>[2x]MAHHHHHHVTSLYKKAGSAAAPFTADTNSNVAVKQINNTGTNDSGEKKVPVPSTNNDSLKQGTDGFWYDSDGNRVDQKTNQILLTAEQLKKNNEKNLSVISDDTSKKDDENISKQTKIANQQTVDTAKGLTTSNLSDPITGGHYENHNGYFVYIDASGKQVTGLQNIDGNLQYFDDNGYQVKGSFRDVNGKHIYFDSVTGKASSNVDIVNGKAQGYDAQGNQLKKSYVADSSGQTYYFDGNGQPLIGLQTIDGNLQYFNQQGVQIKGGFQDVNNKRIYFAPNTGNAVANTEIINGKLQGRDANGNQVKNAFSKDVAGNTFYFDANGVMLTGLQTISGKTYYLDEQGHLRKNYAGTFNNQFMYFDADTGAGKTAIEYQFDQGLVSQSNENTPHNAAKSYDKSSFENVDGYLTADTWYRPTDILKNGDTWTASTETDMRPLLMTWWPDKQTQANYLNFMSSKGLGITTTYTAATSQKTLNDAAFVIQTAIEQQISLKKSTEWLRDAIDSFVKTQANWNKQTEDEAFDGLQWLQGGFLAYQDDSHRTPNTDSGNNRKLGRQPINIDGSKDTTDGKGSEFLLANDID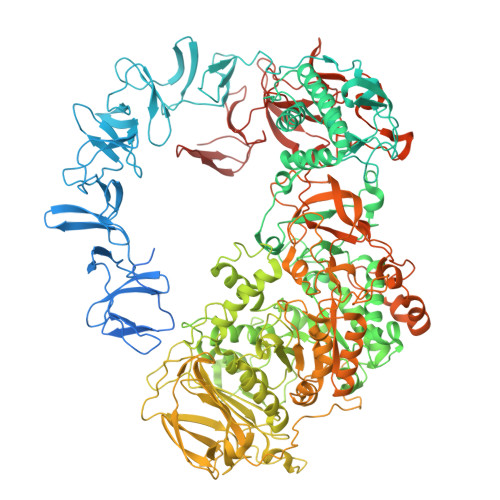NSNPIVQAEQLNWLHYLMNFGSITGNNDNANFDGIRVDAVDNVDADLLKIAGDYFKALYGTDKSDANANKHLSILEDWNGKDPQYVNQQGNAQLTMDYTVTSQFGNSLTHGANNRSNMWYFLDTGYYLNGDLNKKIVDKNRPNSGTLVNRIANSGDTKVIPNYSFVRAHDYDAQDPIRKAMIDHGIIKNMQDTFTFDQLAQGMEFYYKDQENPSGFKKYNDYNLPSAYAMLLTNKDTVPRVYYGDMYLEGGQYMEKGTIYNPVISALLKARIKYVSGGQTMATDSSGKDLKDGETDLLTSVRFGKGIMTSDQTTTQDNSQDYKNQGIGVIVGNNPDLKLNNDKTITLHMGKAHKNQLYRALVLSNDSGIDVYDSDDKAPTLRTNDNGDLIFHKTNTFVKQDGTIINYEMKGSLNALISGYLGVWVPVGASDSQDARTVATESSSSNDGSVFHSNAALDSNVIYEGFSNFQAMPTSPEQSTNVVIATKANLFKELGITSFELAPQYRSSGDTNYGGMSFLDSFLNNGYAFTDRYDLGFNKADGNPNPTKYGTDQDLRNAIEALHKNGMQAIADWVPDQIYALPGKEVVTATRVDERGNQLKDTDFVNLLYVANTKSSGVDYQAKYGGEFLDKLREEYPSLFKQNQVSTGQPIDASTKIKQWSAKYMNGTNILHRGAYYVLKDWATNQYFNIAKTNEVFLPLQLQNKDAQTGFISDASGVKYYSISGYQAKDTFIEDGNGNWYYFDKDGYMVRSQQGENPIRTVETSVNTRNGNYYFMPNGVELRKGFGTDNSGNVYYFDDQGKMVRDKYINDDANNFYHLNVDGTMSRGKGGRADPAFLYKVVSAWSHPQFEK>MASTGVERRKPLENKVALVTASTDGIGLAIARRLAQDGAHVVVSSRKQENVDRTVATLQGEGLSVTGTVCHVGKAEDRERLVAMA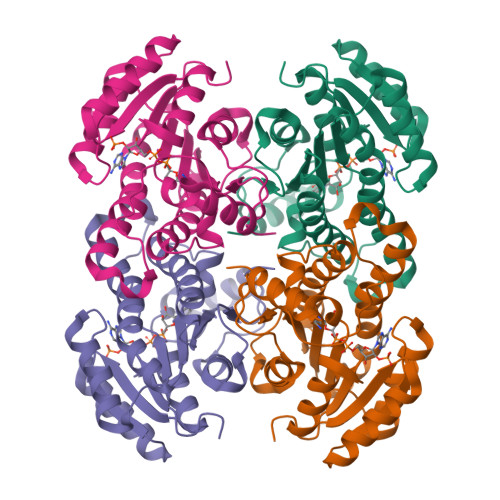VNLHGGVDILVSNAAVNPFFGNIIDATEEVWDKILHVNVKATVLMTKAVVPEMEKRGGGSVLIVSSVGAYHPFPNLGPYNVSKTALLGLTKNLAVELAPRNIRVNCLAPGLIKTNFSQVLWMDKARKEYMKESLRIRRLGNPEDCAGIVSFLCSEDASYITGETVVVGGGTASRL[4x]> APADRLKALVDAAVQPVMKANDIPGLAVAISLKGEPHYFSYGLASKEDGRRVTPETLFEIGSVSKTFTATLAGYALTQDKMRLDDRASQHWPALQGSRFDGISLLDLATYTAGGLPLQFPDSVQKDQAQIRDYYRQWQPTYAPGSQRLYSNPSIGLFGYLAARSLGQPFERLMEQQVFPALGLEQTHLDVPEAALAQYAQGYGKDDRPLRVGPGPLDAEGYGVKTSAADLLRFVDANLHPERLDRPWAQALDATHRGYYKVGDMTQGLGWEAYDWPISLKRLQAGNSTPMALQPHRIARLPAPQALEGQRLLN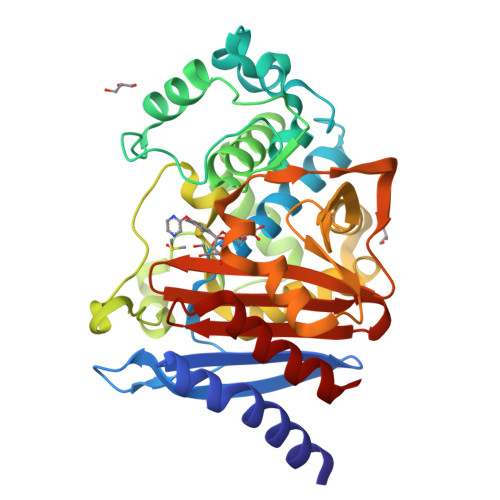KTGSTNGFGAYVAFVPGRDLGLVILANRNYPNAERVKIAYAILSGLE> DSR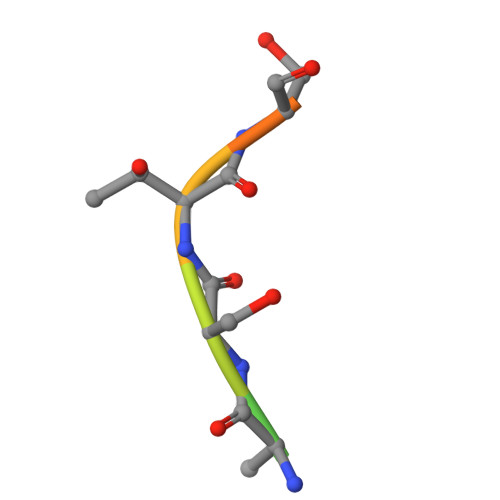ASTSSSS>[16x]MITENEKISLPKIDWALDALEPYISKEINDLHINKHHVAYVNGYNAAIDALEKAVGKRDLKSVVEIQQNIKFHGGGHTNHSLFWKNLAPVSKGGGKHPDTSSALGKQIVAQYG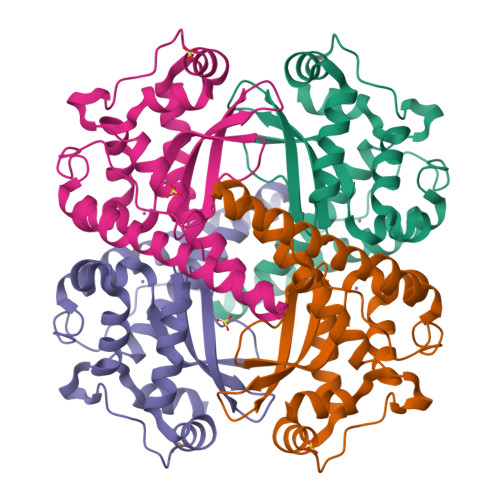SVSNLIDITNSKLAGIQGSGWAFIVKNKQNGGALDVVTTANQDTISAPHLVPIIAIDAWEHAYYLQYQNVRPDYFKAIWNVINWAEAESRYSA>MATLQDIGVSAGINILSAFVFFIIFAVLRLQPFNDRVYFSKWYLKGLRSSPARGGAFAQRFVNLDFRSYMKFLNWMPEALKMPEPELIDHAGLDSVVYLRIYWLGLKIFTPIAVLAWAVLVPVNWTNNTLEMAKQLRNVTSSDIDKLSVSNIPEYSMRFWTHIVMAYAFTIWTCYVLMKEYETIANMRLQFVASEARRPDQFTVLVRNVPPDADESVSELVEHFFLVNHPDHYLTHQVVCNANKLADLVKKKKKLQNWLDYYQLKYARNNSQRIMVKLGFLGLWGQKVDAIEHYIAEIDKISKEISKEREEVVNDPKAIMPAAFVSFKTRWAAAVCAQTQQTRNPTQWLTEWAPEPRDVFWSNLAIPYVSLTVRRLIMHVAFFFLTFFFIVPIAFVQSLATIEGIVKAAPFLKFIVDDKFMKSVIQGFLPGIALKLFLAFLPSILMIMSKFEGFTSISSLERRAAFRYYIFNLVNVFLASVIAGAAFEQLNSFLNQSANQIPKTIGVAIPMKATFFITYIMV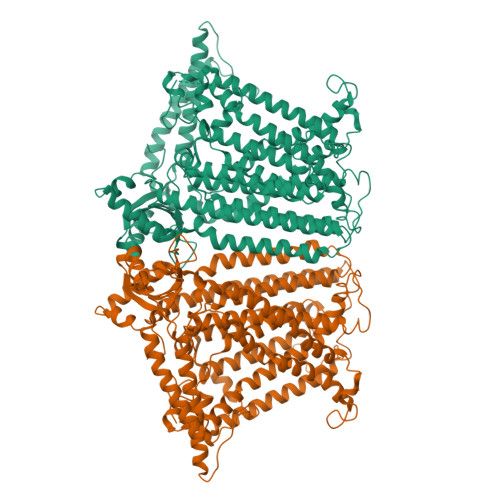DGWAGVAGEILMLKPLIMFHLKNAFLVKTDKDREEAMDPGSIGFNTGEPRIQLYFLLGLVYAPVTPMLLPFILVFFALAYIVYRHQIINVYNQEYESAAAFWPDVHGRVIAALVISQLLLMGLLGTKHAALAAPFLIALPVLTIGFHHFCKGRYEPAFIRYPLQEAMMKDTLETAREPNLNLKGYLQNAYVHPVFKGDEDDYDIDDKLGKFEDEAIIVPTKRQSRRNTPAPSIISGDDSPSLPFSGKLVSNSLEV[2x]>[8x]LEVLDKYSSLIKPKLINNIEAYMVFDKPAHKPNAEAKIYVLLNNHGSRRDIHYKIVSIDRNREVFSKRINVDEKKFLIETISIETPDKPGRFCYKLFIDNEQIDNTCFLVGDPSSREQMYFTIVWHHHQAPNYLPDGRIHGPWAYIYVWSDLLKPYGKGPYHYHSVMLNIHPHFKATYNLSPSLLRQWQIAVEKGVEFVNGEKYDPNHEKIRLVEETLNNYREALFKGQIDVLTSIYAHTIGGFLTDVLGATNIVEEEIRY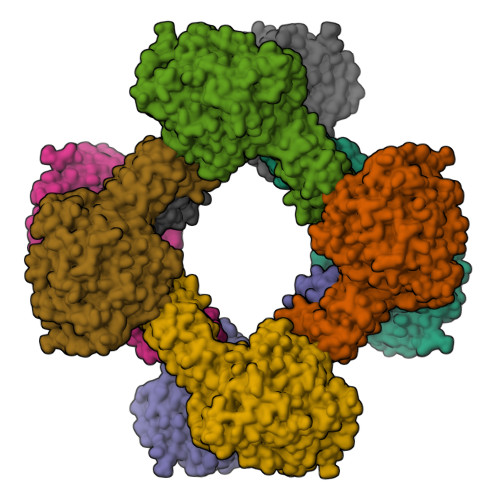GKEVTSKIMGNNYNPQGIWTPEMAFSMKLIPIYYDLDIKYTVLDDKFHFFHAEGNKDSQYEPYMVIDTESKKYITVFFRDHDLSDILGFRNNFYSEPHAWRNAYEFALRVAEKWFDKNVKVLTIALDGENWMSFSVNPPLTAYFLDKMIIYLETLSDNKFIKLSTLREIYNKVPANRILTNIPTNSWLGTFRKWRGEVPQHEEYWIKTYSVYRKLLAYEEMIGGRDEFSNEARWALWHALDSDYWWAEFWLPKIIDTWLSVAENILNNRINKIQIIDVRPASEFYEDEKAGLVVTIRNQLEKEIRVSFAIGGTGFSSVNNDLETVKMNPNSSYTRIIPVKAKFIGKHKMVVSAISKGLIIDSKIIDINVKPKLLPNPRLEHHHHHH>AVGPVADLTVTNANIVPDGFERAAIVVNNVFPAPLITGNMGDNFQLNLVNQMTNHTMLKTTSIHWHGFFQKGTNWADGPAFINQCPIASGNSFLYDFQVPGQAGTFWYHSHLSTQYCDGLRGPFVVYDPNDPHANLYDVDDESTVITLADWYHVAAKLGPRFPKGADSTLINGLGRSTSTPTADLAVISVTKGKRYRFRLVSLSCDPNYTFSIDSHQLTVIEADGVSTQPVTVDSIQIFAAQRYSFVLNANQDVDNYWIRANPNFGTTGFADGVNSAILRYDDADPVEPVTNQTGTTLLLETDLHPLTSMPVPGNPTQGGADLNLNMAFNFDGTNFFINGESFTPPTVPVLLQIISGANTAQDLLPSGSVYSLPSNSSIEITFPATTAAPGAPHPFHLHGHVFAVVRSAGSTSYNYDDPVWRDVVSTGTPQAGDNVTIRFQTDNPGPWFLHCHIDFHLDAGFAVVMAEDIPNTVNANPVPQAWSNLCPTYDALEPSNE[2x]

Laccases belong to multicopper oxidases, a widespread class of enzymes implicated in many oxidative functions in pathogenesis, immunogenesis and morphogenesis of organisms and in the metabolic turnover of complex organic substances. They catalyze the coupling between the four one-electron oxidations of a broad range of substrates with the four-electron reduction of dioxygen to water.

The structure of the blue laccase, a multicopper oxidase from the white-rot basidiomycete fungus Lentinus (Panus) tigrinus, involved in lignin and xenobiotics biodegradation, was solved at 1.5 Å. It exhibits a molecular architecture organized in three sequentially arranged cupredoxin-like domains; each of them has a greek key β-barrel topology, strictly related to the small copper proteins like azurin and plastocyanin and common to all the members of the blue multicopper oxidase family, like the ascorbate oxidase and the mammalian ceruloplasmin. Of the six putative N-glycosylation sites (consensus sequence N-X-T/S) only at Asn54, Asn376, and Asn435 the density maps indicate the presence of glycosilaytion. The structure is further stabilized by two sulphur bridges, one between Cys85 and Cys487 from domains 1 and 3 respectively and the other between Cys117 and Cys 205 from domains 1 and 2 correspondingly. The T1 copper ion (occupancy 0.75) presents a planar triangular coordination with two histidine (His394 and His457) and one cysteine (Cys452) residues. Exposing LtL crystals at pH 8.5 to high X-rays radiation doses under aerobic condition allowed us to detect two intermediates in the catalyzed molecular oxygen splitting, most likely corresponding to the 2-electrons and 4-electrons reduction stages. The electron-density maps from LtL disclosed two different T2/T3 cluster-dioxygen arrangements in the two laccase molecules (A and B) present into the asymmetric unit, possibly corresponding to two different reduction states of the oxygen molecule along the reduction pathway. In both molecules the T2 copper center is coordinated to His64, His397 and one OH- ligand whereas the T3 copper centers are coordinated to 3 histidine residues each (His111, His399, and His451 for T3(a), His66, His109, and His453 for T3(b)). It should be noted that differences observed among the structural data of multicopper oxidases published to date, and acquired using synchrotron radiation, are difficult to interpret since they most probably represent pictures of the copper sites resulting from the average of the starting oxidized state and of the partially/totally reduced coppers/dioxygen adduct states and strictly reliant on the acquired x-ray doses and on the other experimental conditions.> DAGDKGIYRHYMQKEIYEQPNAIKNTLTGRISHGQVDLSELGPNADELLSKVEHIQILACGTSYNSGMVSRYWFESLAGIPCDVEIASEFRYRKS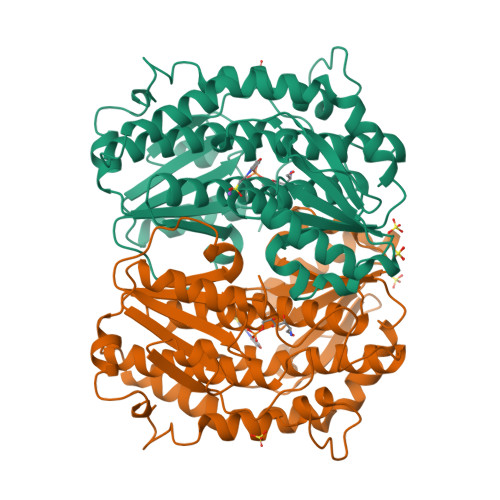AVRRNSLMITLSQSGETADTLAGLRLSKELGYLGSLAICNVPGSSLVRESDLALMTNAGTEIGVASTKAFTTQLTVLLMLVAKLSRLKGLDASIEHDIVHGLQALPSRIEQMLSQDKRIEALAEDFSDKHHALFLGRGDQYPIALEGALKLKEISYIHAEAYAAGELKHGPLALIDADMPVIVVAPNNELLEKLKSNIEEVRARGGQLYVFADQDAGFVSSDNMHIIEMPHVEEVIAPIFYTVPLQLLAYHVALIKGTDVDQPRNLAKSVTVE> MAHHHHHHHHHHSGRELQPPEASIAVVSIPRQLPGSHSEAGVQGLSAGDDSETGSDCVTQAGLQLLASSDPPALASKNAEVTVETGFHHVSQADIEFLTSIDPTASASGSAGITGTMSQDTEVDMKEVELNELEPEKQPMNAASGAAMSLAGAEKNGLVKIKVAEDEAEAAAAAKFTGLSKEELLKVAGSPGWVRTRWALLLLFWLGWLGMLAGAVVIIVRAPRCRELPAQKWWHTGALYRIGDLQAFQGHGAGNLAGLKGRLDYLSSLKVKGLVLGPIHKNQKDDVAQTDLLQIDPNFGSKEDFDSLLQSAKKKSIRVILDLTPNYRGENSWFSTQVDTVATKVKDALEFWLQAGVDGFQVRDIENLKDASSFLAEW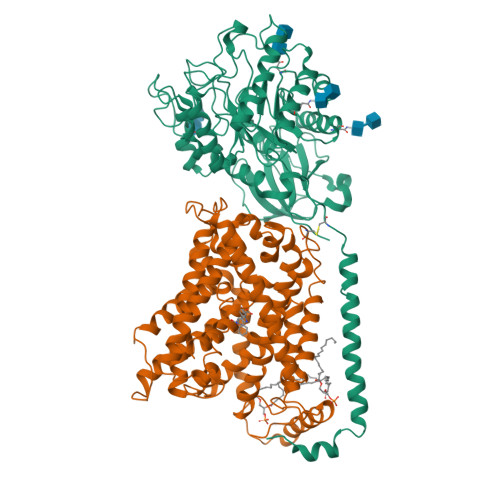QNITKGFSEDRLLIAGTNSSDLQQILSLLESNKDLLLTSSYLSDSGSTGEHTKSLVTQYLNATGNRWCSWSLSQARLLTSFLPAQLLRLYQLMLFTLPGTPVFSYGDEIGLDAAALPGQPMEAPVMLWDESSFPDIPGAVSANMTVKGQSEDPGSLLSLFRRLSDQRSKERSLLHGDFHAFSAGPGLFSYIRHWDQNERFLVVLNFGDVGLSAGLQASDLPASASLPAKADLLLSTQPGREEGSPLELERLKLEPHEGLLLRFPYAALE;> MADYKDDDDKSGPDEVDASGREEGARHRNNTEKKHPGGGESDASPEAGSGGGGVALKKEIGLVSACGIIVGNIIGSGIFVSPKGVLENAGSVGLALIVWIVTGFITVVGALCYAELGVTIPKSGGDYSYVKDIFGGLAGFLRLWIAVLVIYPTNQAVIALTFSNYVLQPLFPTCFPPESGLRLLAAICLLLLTWVNCSSVRWATRVQDIFTAGKLLALALIIIMGIVQICKGEYFWLEPKNAFENFQEPDIGLVALAFLQGSFAYGGWNFLNYVTEELVDPYKNLPRAIFISIPLVTFVYVFANVAYVTAMSPQELLASNAVAVTFGEKLLGVMAWIMPISVALSTFGGVNGSLFTSSRLFFAGAREGHLPSVLAMIHVKRCTPIPALLFTCISTLLMLVTSDMYTLINYVGFINYLFYGVTVAGQIVLRWKKPDIPRPIKINLLFPIIYLLFWAFLLVFSLWSEPVVCGIGLAIMLTGVPVYFLGVYWQHKPKCFSDFIELLTLVSQKMCVVVYPEVERGSGTEEANEDMEEQQQPMYQPTPTKDKDVAGQPQP>[2x]SNAMSLLARLEQSVHENGGLIVSCQPVPGSPMDKP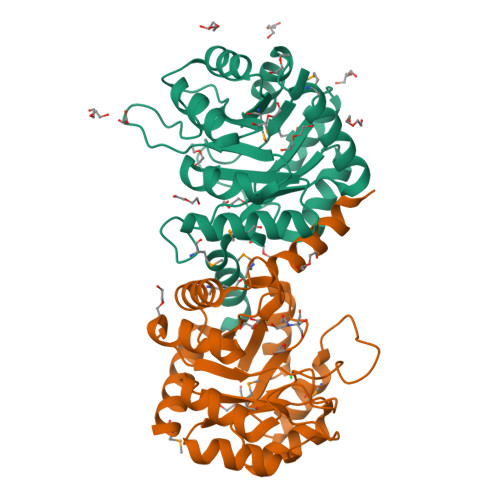EIVAAMAQAAASAGAVAVRIEGIENLRTVRPHLSVPIIGIIKRDLTGSPVRITPYLQDVDALAQAGADIIAFDASFRSRPVDIDSLLTRIRLHGLLAMADCSTVNEGISCHQKGIEFIGTTLSGYTGPITPVEPDLAMVTQLSHAGCRVIAEGRYNTPALAANAIEHGAWAVTVGSAITRIEHICQWFSHAVKR> SN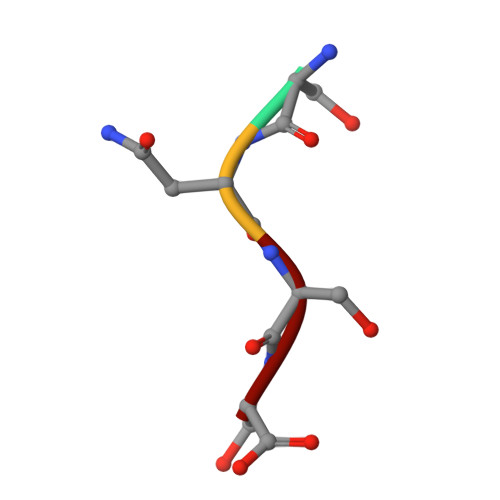SS>[18x]HHHHHHMKTRIHVVQGDI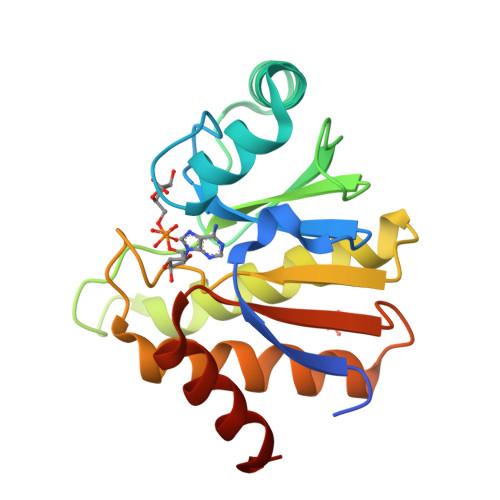TKLAVDVIVNAAAPSLMGGGGVAGAIHRAAGPALLDACLKVRQQQGDCPTGHAVITLAGDLPAKAVVHTVGPVWRGGEQNEDQLLQDAYLNSLRLVAANSYTSVAFPAISTGVYGYPRAAAAEIAVKTVSEFITRHALPEQVYFVCYDEENAHLYERLLTQQGDE>[2x]MGSLVCVGTGLQLAGQISVLSRSYIEHADIVFSLLPDGFSQRWLTKLNPNVINLQQFYAQNGEVKNRRDTYEQMVNAILDAVRAGKKTVCALFGHPGVFACVSHMAITRAKAEGFSAKMEPGISAEACLWADLGIDPGNSGHQSFEASQFMFFNHVPDPTTHLLLWQIAIAGEHTLTQFHTSSDRLQILVEQLNQWYPLDHEVVIYEAANLPIQAPRIERLPLANLPQAHLMPISTLLIPPAKKLEYNYAILAKLGIGPEDLG;>[2x]MSGLSDFFTQLGQDAQLMEDYKQNPEAVMRAHGLTDEQINAVMTGDMEKLKTLSGDSSYQSYLVISHGNGD

Here we report the discovery of type IV borosin natural product pathways (termed ‘split borosins’), featuring an iteratively acting α-N-methyltransferase and separate precursor peptide substrate from the metal-respiring bacterium Shewanella oneidensis. The α-N-methyltransferase SonM from Shewanella oneidensis MR-1 iteratively methylates its substrate SonA at two residues, SonA-L63 and SonA-I65, in an N-to-C terminal fashion on the core peptide. Complexes of SonM and SonA form dimers of heterodimers. A five helical bundle at the N-terminus of SonA, now referred to as the borosin binding domain (BBD; 1–53), serves as the SonA leader peptide and is homologous to a portion of the fused clasp region of OphMA.

Among the mutations targeting residues directly interacting with the core peptide, SonM-Y93F shows the smallest changes in catalytic efficiency, as compared to the wt enzyme. However, the mutant exhibits the largest change in the apparent KM value for SAM (220 μM, a 3.8-fold increase as compared to wt). While, globally, the SonM-Y93F mutant structure complex does not reveal significant differences to wt, the structural observation that mutation of SonM-Y93 incurs a conformational change upon SAH binding is consistent with the increased apparent KM value and a role in binding SAM. Consequently, the cofactor cavity is significantly larger, and the ability of SonM-Y93 to switch between an inward trajectory towards the cofactor and outwards towards solvent and suggests a role in cofactor binding and release. This structural data corroborates the increase in the apparent KM of SAM for the SonM-Y93F mutant.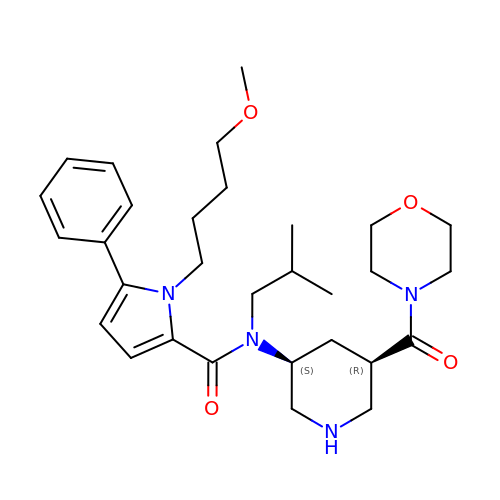1-(4-methoxybutyl)-N-(2-methylpropyl)-N-[(3S,5R)-5-(morpholine-4-carbonyl)piperidin-3-yl]-5-phenyl-1H-pyrrole-2-carboxamide | C30 H44 N4 O4 | URICGOHQZDVMJG-FTJBHMTQSA-N> MEALGINPTLFIAQLINFLLLIFILRALLYRPVMNLLNERTRRIEESVRDAEKVREQLANARRDYEAEIARARQEAAKIVAQAQERAKQQEAEIIAQARREAER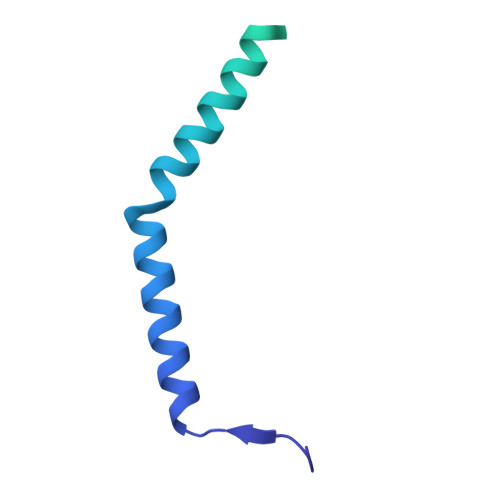LKEEARAQAEQERIRMLSEAKSQIADLVTLTASRVLGAELQARGHDALIAESLAALDRRN>[2x]MDSKHQCVKLNDGHFMPVLGFGTYAPPEVPRSKALEVTKLAIEAGFRHIDSAHLYNNEEQVGLAIRSKIADGSVKREDIFYTSKLWSTFHRPELVRPALENSLKKAQLDYVDLYLIHSPMSLKPGEELSPTDENGKVIFDIVDLCTTWEAMEKC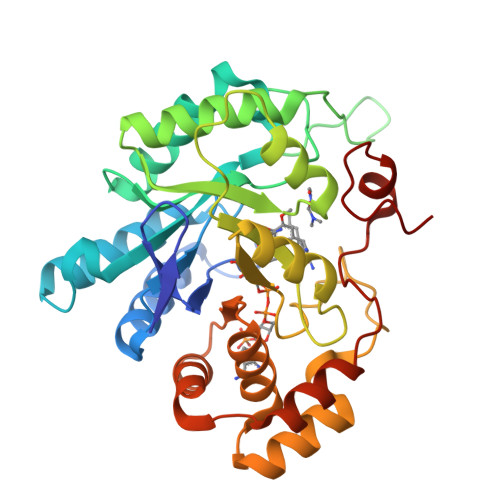KDAGLAKSIGVSNFNRRQLEMILNKPGLKYKPVCNQVECHPYFNRSKLLDFCKSKDIVLVAYSALGSQRDKRWVDPNSPVLLEDPVLCALAKKHKRTPALIALRYQLQRGVVVLAKSYNEQRIRQNVQVFEFQLTAEDMKAIDGLDRNLHYFNSDSFASHPNYPYSDEY>[2x]VSFRQKRTRIPLLAMTVTALAAAVCGVTTAPAATGAEVAVPLSVGAAAGNATPIPGYVIQSSAQVSDDSAVSKPGFPTSGWYPVSSRSTVYAGLLQNGKYADPFYSTNMQNVPAAQFSVPWWYRTDLNVDDTSSRTYLDFSGVLSKADVWVNGTKVATKDQVNGAYTRHDLDITAQVHTGVNSVAFKVYPNDPNRDLSMGWIDWAQTPPDQNMGIVRDVLVRRSGAVALRSAHVIQKLNSALDHADLTVKADVRNDSANAVQTTVAGTVAGKPISQTVSLAAKERKTVTFPLVGLDRPNVWWPAGMGGQHRYDLDLTASVGGTPSDAAKSKFGVRDVKATLNSSGGRQYSVNGKPLLIRGGGYTPDLFLRWNETAAADKLKYVLNLGLNTVRLEGHIEPDEFFDIADDLGVLTMPGWECCDKWEGQVNGEEKGEPWVESDYPIAKASMFSEAERLRDHPSVISFHIGSDFAPDRRIEQGYLDAMKAADFLLPVIPAASARPSPITGASGMKMNGPYDYVPPVYWYDKSQKDRGGAWSFNSETSAGVDIPTMDTLKRMMSASELDTMWKNPSAKQYHRSSSDTFGNLKLFGDALTKRYGASANLNDFVRKAQLSQYENVRAEFESHSRNYTDSTNPSTGLIYWMLNSPWTSLHWQLFDAYMDQNGAYYGAKKANEPLHIQYSHDNRSVVVINQTSNAVSGLTATTKLYNLDGTEKYSNTKTGLSVGALGAKATAVTVPAVSGLSTTYLAKNVLTDSSGKEVSRNVYWLSTKADTLNWGGSDWYYTPQSAFADLSGLNNLGQSAVGATANSVAGADGTTTTTVTLKNTSGGRLPAFYVDSKVVDSAGKPVLPVEWNDNAVSLWPGETTTLTAKYRTADLKGSKPSVRISGWNTGTQTVPADGSGPGPSDPVDYQAEDATIVQGAVESNHAGYTGTGFVNYDNVAGSSVEWTVTVPSAGTYD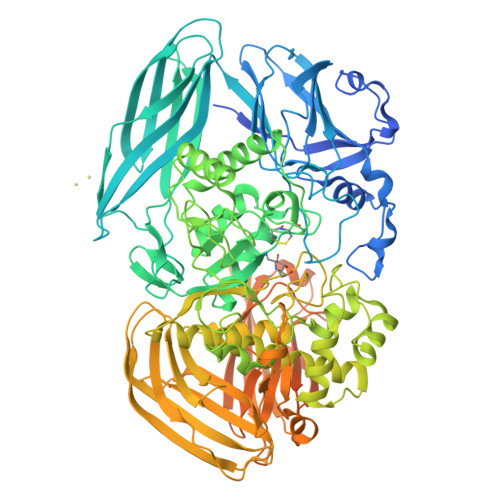VVVRYANGTTTSRPLDFSVNGSISASGVAFGSTGTWPAWTTKTVRVTLAAGVNKIKAVATTANGGPNVDKITL>[5x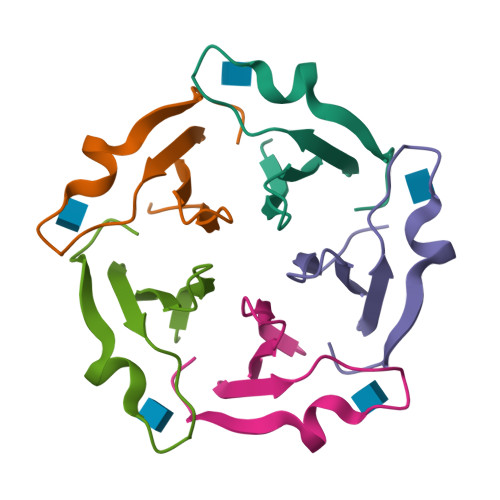]MSGFKFLFFSPDGTLYGVHNDKLYKGTPPTSDKDNWLARATLIGNGGW> MAPARPNWLAYDWGLVFLVAAIVALGFVNLGSAAPDPVLLYRQSVALGLGLLLAFLLQFLSRRRLFGLAYPLYGASLLLLALVLVVGREINGARAWFVLGPLQFQPLELAKLGLLLALAKALEGRPIARVWDYALPALLTLPVVGLLLLQPDLGGALVVLFGVFVVVFVRGLPWRHLLVGLFALALLVPTAVWPNLKPYQRERVLIVLDPYRDPLGQGFQVIQSTIAIGSGGLFGKGYGQGTQAQLGFIPFRHTDFVFSVWAEEWGFVGVVGLLGLYGLLLARLFALALACPRLSDRLFL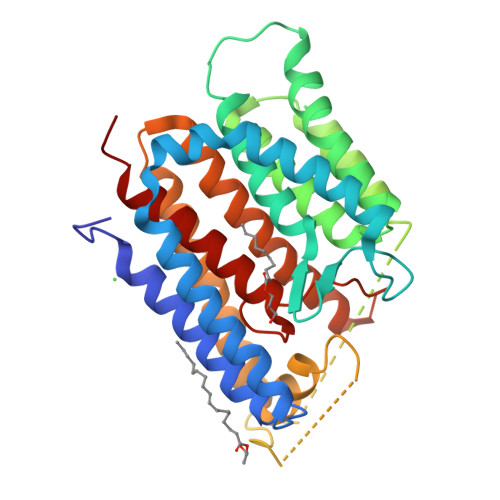SGFAGMLGFQVVVNLGVALGVMPVTGLTLPLFSYGGSSLIATLAGLGLVLLVHRDRYQD>[2x]GSRNQSPPQMMAQQGMHMQWTDQSFIEMMTPHHQDAIDMAEMALQKAEHPELKK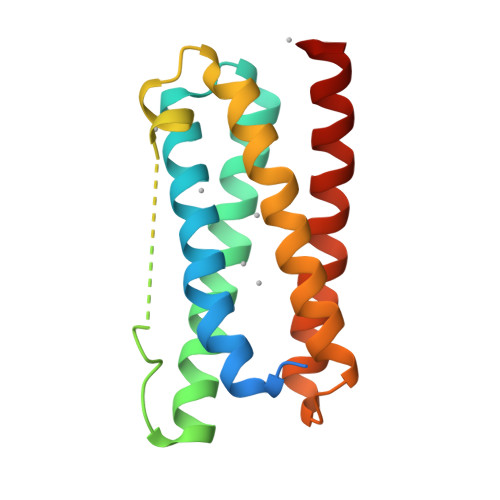LARNIIRDQEREIKEMKTWYQQWFKRPVPALSSQGMMGMHQGHGMMAMDLDALATAQNFDREFIRQMIPHHQMAVMMASNLKTNTERPEMDKLMDDIIRSQSAEIKQMKQWYQNWYGQ> KCTVSHEVADCSHLKLTQVPDDLPTNITVLNLTHNQLRRLPAANFTRYSQLTSLDVGFNTISKLEPELCQKLPMLKVLNLQHNELSQLSDKTFAFCTNLTELHLMSNSIQKIKNNPFVKQKNLITLDLSHNGLSSTKLGTQVQLENLQELLLSNNKIQALKSEELDIFANSSLKKLELSSNQIKEFSPGCFHAIGRLFGLFLNNVQLGPSLTEKLCLELANTSIRNLSLSNSQLSTTSNTTFLGLKWTNLTMLDLSYNNLNVVGNDSFAWLPQLEYFFLEYNNIQHLFSHSLHGLFNVRYLNLKRSFTKQSISLASLPKIDDFSFQWLKCLEHLNMEDNDIPGIKSNMFTGLINLKYLSLSNSFTSLRTLTNETFVSLAHSPLHILNLTKNKISKIESDAFSWLGHLEVLDLGLNEIGQELTGQEWRGLENIFEIYLSYNKYLQLTRNSFALVPSLQRLMLRRVALKNVDSSPSPFQPLRNLTILDLSNNNIANINDDMLEGLEKLEILDLQHNNLARLWKHANPGGPIYFLKGLSHLHILNLESNGFDEIPVEVFKDLFELKIIDLGLNNLNTLPASVFNNQVSLKSLNLQKNLITSVEKKVFGPAFRNLTELDMRFNPFDCTCESIAWFVNWINETHTNIPELSSHYLCNTPPHYHGFPVRLFDTSSCKDSA;> SLEEEAERVVEELVKEFNLSRTQEIALRRYAEYAARATASEEVIEELLRDVAERLS

Toll-like Receptor 3 (TLR3) is a pattern recognition receptor that initiates antiviral immune responses upon binding double-stranded RNA (dsRNA). The extracellular domain is responsible for ligand recognition and contains multiple leucine-rich repeats (LRRs) that form a horseshoe-like structure. Here, we use computational protein design to create novel miniproteins that bind to human TLR3 with nanomolar affinities. Cryo-EM structures of two minibinders in complex with TLR3 reveal that they bind the target as designed, although one partially unfolds due to steric competition with a nearby N-linked glycan.

Following a strategy previously established for structural characterization of TLR4/MD-2 complexes, we co-expressed the TLR3 ectodomain and each minibinder in HEK293F cells and co-purified the complexes using affinity chromatography followed by SEC. This improved occupancy, and after optimizing grid preparation and data collection to overcome a clear preferred orientation, we determined cryo-EM structures of minibinders 7.7 and 8.6 in complex with TLR3, each at 2.9 Å resolution. Minibinders 7.7 and 8.6 interacted with the concave surface of TLR3 in slightly different manners, with α1 and α2 of minibinder 7.7 binding to LRR15-LRRCT and α2 and α3 of minibinder 8.6 binding to LRR13-LRRCT. Hydrophobic residues on both minibinders (7.7: M3, Y6, L35, V36, and I39; 8.6: Y30, Y33, A34, V43, L47, and V51) form hydrophobic networks with I510, I534, I566, and I590 in Site A of TLR3 as intended. Conversely, minibinder 8.6 maintained a stable 3-helical bundle through core hydrophobic interactions. In contrast to minibinder 7.7, the electrostatic interactions mediated by Y33 and conserved residues (R29, Y30, K/R36, E42, E46) in minibinder 8 and its derivatives surround a hydrophobic core interaction network in the minibinder 8.6/TLR3 complex. Interestingly, our structural analysis revealed that the interaction of T38 with A35 and I44 stabilizes the loop connecting α2 and α3, facilitating the formation of hydrogen bonds between S40 and E42 of minibinder 8.6 and E639 and N667 of TLR3, respectively. Additionally, the R50D substitution in minibinder 8.6 enabled the formation of an ionic interaction with K589 of TLR3. These observations likely explain why the G38T and R50D substitutions significantly enhanced the binding affinity of minibinder 8.6 compared to 8.4. When the cryo-EM structures were superimposed on the AlphaFold2-predicted models of each complex, the Cα RMSDs between minibinders 7.7 and 8.6 and their predictions were 1.0 and 2.0 Å, respectively. For minibinder 8.6, the α2 and α3 helices were well-aligned (Cα RMSD: 1.6 Å), but α1 was slightly displaced from its predicted position (Cα RMSD: 2.7 Å).> GAMDPKVTMNDFDYLKLLGKGTFGKVILVREKATGRYYAM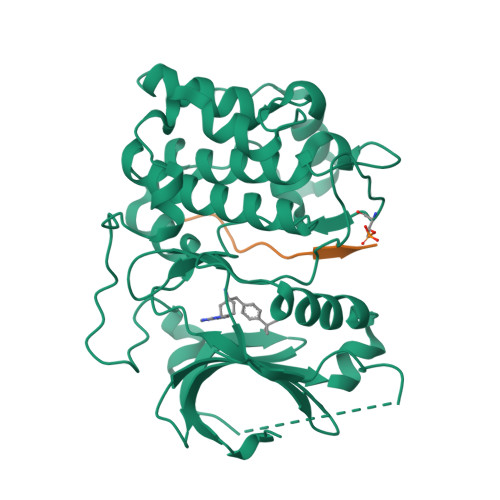KILRKEVIIAKDEVAHTVTESRVLQNTRHPFLTALKYAFQTHDRLCFVMEYANGGELFFHLSRERVFTEERARFYGAEIVSALEYLHSRDVVYRDIKLENLMLDKDGHIKITDFGLCKEGISDGATMKTFCGTPEYLAPEVLEDNDYGRAVDWWGLGVVMYEMMCGRLPFYNQDHERLFELILMEEIRFPRTLSPEAKSLLAGLLKKDPKQRLGGGPSDAKEVMEHRFFLSINWQDVVQKKLLPPFKPQVTSEVDTRYFDDEFTAQSITITPPDRYDSLGLLELDQREEQEMFEDFDYIADW;> GRPRTTSFAE> MDEKLLKTIAESKYLVALTGAGVSAESGIPTFRGKDGLWNRYRPEELANPQAFAKDPEKVWKWYAWRMEKVFNAQPNKAHQAFAELERLGVLKCLITQNVDDLHERAGSRNVIHLHGSLRVVRCTSCNNSFEVESAPKIPPLPKCDKCGSLLRPGVVWFGEMLPPDVLDRAMREVERADVIIVAGTSAVVQPAASL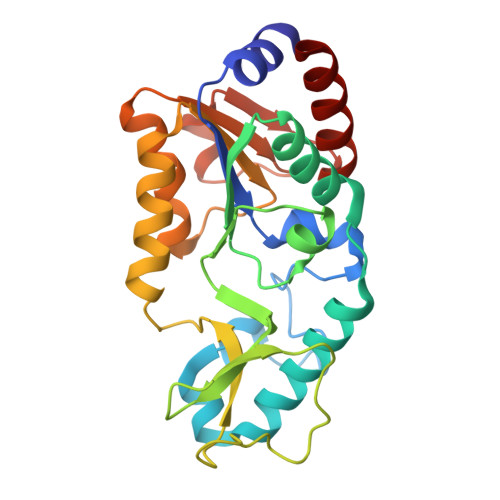PLIVKQRGGAIIEINPDETPLTPIADYSLRGKAGEVMDELVRHVRKALS> MKRVMFHAKIHRATV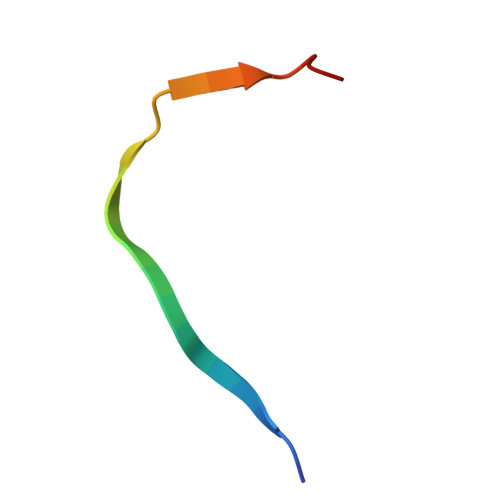TQADLHYVG>[7x]RKENELLRREKDLKEEEYVFESPKMKEILEKIKKISCAECPVLITGESGVGKEVVARLIHKLSDRSKEPFVALNVASIPRDIFEAELFGYEKGAFTGAVSSKEGFFELADGGTLFLDAIGELSLEAQAKLLRVIESGKFYRLGGRKEIEVNVRILAATNRNIKELVKEGKFREDLYYRLGVIEIEIPPLRERKEDIIPLANHFLKKFSRKYAKEVEGFTKSAQELLLSYPWYGNVRELKNV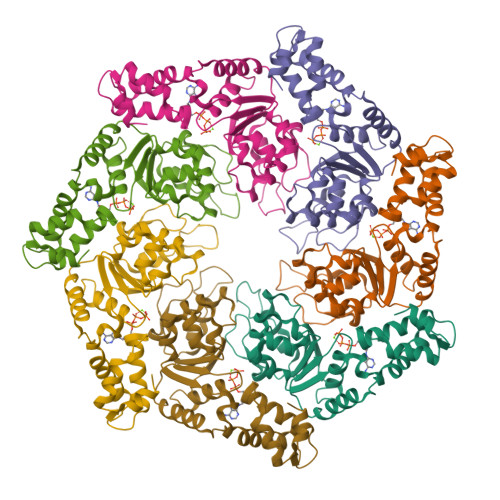IERAVLFSEGKFIDRGELSCLVNSK>[4x]MEYEWKPDEQGLQQILQLLKESQSPDTTIQRTVQQKLEQLNQYPDFNNYLIFVLTKLKSEDEPTRSLSGLILKNNVKAHFQNFPNGVTDFIKSECLNNIGDSSPLIRATVGILITTIASKGELQNWPDLLPKLCSLLDSEDYNTCEGAFGALQKICEDSAEILDSDVLDRPLNIMIPKFLQFFKHSSPKIRSHAVACVNQFIISRTQALMLHIDSFIENLFALAGDEEPEVRKNVCRALVMLLEVRMDRLLPHMHNIVEYMLQRTQDQDENVALEACEFWLTLAEQPICKDVLVRHLPKLIPVLVNGMKYSDIDIILLKGDVEEDETIPDSEQDIRPRFHRSRTVAQQHDEDGIEEEDDDDDEIDDDDTISDW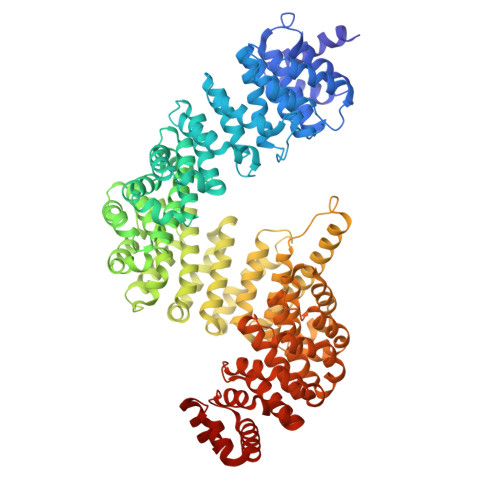NLRKCSAAALDVLANVYRDELLPHILPLLKELLFHHEWVVKESGILVLGAIAEGCMQGMIPYLPELIPHLIQCLSDKKALVRSITCWTLSRYAHWVVSQPPDTYLKPLMTELLKRILDSNKRVQEAACSAFATLEEEACTELVPYLAYILDTLVFAFSKYQHKNLLILYDAIGTLADSVGHHLNKPEYIQMLMPPLIQKWNMLKDEDKDLFPLLECLSSVATALQSGFLPYCEPVYQRCVNLVQKTLAQAMLNNAQPDQYEAPDKDFMIVALDLLSGLAEGLGGNIEQLVARSNILTLMYQCMQDKMPEVRQSSFALLGDLTKACFQHVKPCIADFMPILGTNLNPEFISVCNNATWAIGEISIQMGIEMQPYIPMVLHQLVEIINRPNTPKTLLENTAITIGRLGYVCPQEVAPMLQQFIRPWCTSLRNIRDNEEKDSAFRGICTMISVNPSGVIQDFIFFCDAVASWINPKDDLRDMFCKILHGFKNQVGDENWRRFSDQFPLPLKERLAAFYGV> GLVPRGSHMAGAQDFVPHTADLAELAAAAGECRGCGLYRDATQAVFGAGGRSARIMMIGEQPGDKEDLAGLPFVGPAGRLLDRALEAADIDRDALYVTNAVKHFKFTRAAGGKRRISKTPSRTEVVACRPWLIAEMTSVEPDVVVLLGATAAKALLGNDFRVTQHRGEVLHVDDVPGDPALVATVHPSSLLAGPKEERESAFAGLVDDLRVAADV

UdgX excises uracil from uracil-containing DNA to concurrently form a covalent bond with the resulting AP-DNA. Structurally, UdgX is highly similar to family-4 UDGs (F4-UDGs). However, UdgX is unique in possessing a flexible R-loop (105KRRIH109). Our earlier studies allowed us to propose a reaction mechanism of UdgX, which involves the formation of a covalent bond between H109 of UdgX with the C1′ position of the target deoxyribose sugar concurrently with the uracil excision from this site in DNA.

Furthermore, based on our structural analyses, we suggested that R184 in the DNA intercalation loop (motif B) facilitates localization of the target U in the active site. The R184A mutation (motif B) supports the role of R184 in substrate-binding. We combined H109S and R184A mutations and measured the kinetics of uracil excision. H109S/R184A mutant showed nearly 2-fold increase in its Km as compared to H109S, and about 4-fold decrease in Kcat/Km. To understand this further, we determined the structure of H109S/R184A mutant and compared the R184A region of it with the structure of UdgX–DNA complex. The NG and NE of R184 established H-bonds of 3.53 and 3.55 Å lengths with the phosphate backbone of DNA (P + 1), and the NE of R184 makes another hydrogen bond with (P – 1) of DNA backbone with 2.32 Å distance. These observations emphasise the role of R184 in binding of DNA substrate with UdgX. In addition, our biochemical and structural analysis of the R184 mutant shows that R184 is critical in binding to the DNA by establishing multiple interactions with the phosphate backbone in the neighbourhood of the uracil in the DNA. The R184A mutation results in ∼2-fold increase in Km for DNA binding and an overall reduction of ∼4 fold in Kcat/Km value of the mutant confirming its role in stabilization of the enzyme substrate complex.>QVVSQG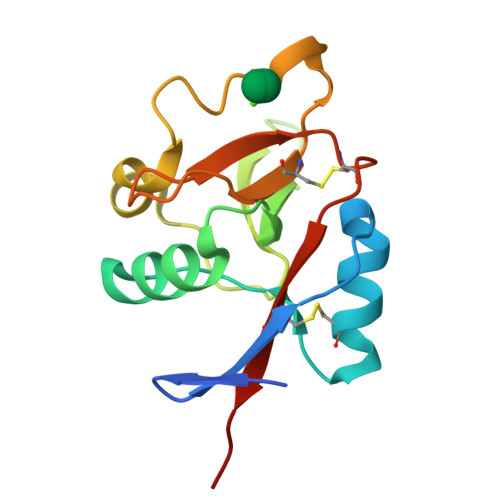WKYFKGNFYYFSLIPKTWYSAEQFCVSRNSHLTSVTSESEQEFLYKTAGGLIYWIGLTKAGMEGDWSWVDDTPFNKVQSARFWIPGEPNNAGNNEHCGNIKAPSLQAWNDAPCDKTFLFICKRPYVPSEP[4x]Herewith, the bridging enzyme PfAldolase, which binds actin in addition to its role in glycolysis, plays a key role: it connects the actin/myosin motor to trans-membrane adhesins of the thrombospondin-related anonymous protein (TRAP) family, which are expressed in a life-cycle stage specific manner. The cleavage reaction leaves the extracellular TRAP domains bound to the host cell or substrate, while the cytoplasmic C-termini, also referred to as TRAP-tails, remain bound to PfAldolase, from which they are believed to dissociate and be recycled for degradation over time. TRAP is a competitive inhibitor of PfAldolase as the binding sites of the glycolytic substrate fructose 1,6-bisphosphate (F16BP) and TRAP partially overlap.

While traditional, targeted inhibitor-design approaches are usually geared towards finding small molecules that prevent protein–protein interactions (PPI) critical to the pathogen, the hypothesis explored here is counter-intuitive: strengthening, instead of hindering, the PfAldolase–TRAP interaction is hypothesized to inhibit motility and invasion. Finally, the ternary co-crystal structure of PfAldolase–TRAP with compound 24 stabilizing the interaction was determined. However in only one case, that of compound 24, clear electron density was observed for both TRAP and the compound in all four sub-units of the aldolase tetramer. Overall, the TRAP-tails are pushed further into the pocket of aldolase upon addition of the small molecule stabilizer, compound 24, thereby occluding the F16P substrate-binding site. The W604 ring system varies only slightly in its position by 0.8 Å, whereas the D603 Ca-position shifts by 3.6 Å and the N605 Ca-position by 4.7 Å. The dihydroxybenzyl-ring of compound 24 stays within the experimental error of the X-ray crystal structure in the same position in all four sub-units, contacting residue N606 of TRAP and N39, E40, T44 of aldolase through hydrophobic interactions. The dichlorobenzyl-ring system adopts two major conformations, indicating flexibility of the compound when bound to the PfAldolase–TRAP interface. The contacting residues on aldolase mainly provide hydrophobic interactions mediated through residues L117, R158 and L198 for binding mode 1 and T44, K47 and R48 in the alternative conformation, while also contacting D604 of the TRAP-tail. While compound 24 did not induce a significant change in activity in the rabbit aldolase or PfAldolase alone, a dramatic change in activity was observed upon addition of both the TRAP-peptide and compound 24 to PfAldolase, further supporting the initial hypothesis of compound 24 acting as a stabilizing agent of the PfAldolase–TRAP protein–protein interaction. The association constant (Ka) decreases and the dissociation rate (Kd) increases in the presence of compound 24, thereby indicating a stabilizing effect on the PfAldolase–TRAP complex under physiological buffer conditions.

>MAHCTEYMNAPKKLPADVAEELATTAQKLVQAGKGILAADESTQTIKKRFDNIKLENTIENRASYRDLLFGTKGLGKFISGAILFEETLFQKNEAGVPMVNLLHNENIIPGIKVDKGLVNIPCTDEEKSTQGLDGLAERCKEYYKAGARFAKWRTVLVIDTAKGKPTDLSIHETAWGLARYASICQQNRLVPIVEPEILADGPHSIEVCAVVTQKVLSCVFKALQENGVLLEGALLKPNMVTAGYECTAKTTTQDVGFLTVRTLRRTVPPALPGVVFLSGGQSEEEASVNLNSINALGPHPWALTFSYGRALQASVLNTWQGKKENVAKAREVLLQRAEANSLATYGKYKGGAGGENAGASLYEKKYVY[4x];> AASLYEKKAA;> AAASLYEKKAA;>[4x]DWN>NNNFFDPKLMSDWEDEDLDTDNDNIPDSYERNGYTIKDLIAVKWEDSFAEQGYKKYVSNYLESNTAGDPYTDYEKASGSFDKAIKTEARDPLVAAYPIVGVGMEKLIISTNEHASTDQGKTVSRATTNSKTESNTAGVSVNVGYQNGFTANVTTNYSHTTDNSTAVQDSNGESWNTGLSINKGESAYINANVRYYNTGTAPMYKVTPTTNLVLDGDTLSTIKAQENQIGNNLSPGDTYPKKGLSPLALNTMDQFSSRLIPINYDQLKKLDAGKQIKLETTQVSGNFGTKNSSGQIVTEGNSWSDYISQIDSISASIILDTENESYERRVTAKNLQDPEDKTPELTIGEAIEKAFGATKKDGLLYFNDIPIDESCVELIFDDNTANKIKDSLKTLSDKKIYNVKLERGMNILIKTPTYFTNFDDYNNYPSTWSNVNTTNQDGLQGSANKLNGETKIKIPMSELKPYKRYVFSGYSKDPLTSNSIIVKIKAKEEKTDYLVPEQGYTKFSYEFETTEKDSSNIEITLIGSGTTYLDNLSITELNSTPEILDEPEVKIPTDQEIMDAHKIYFADLNFNPSTGNTYINGMYFAPTQTNKEALDYIQKYRVEATLQYSGFKDIGTKDKEMRNYLGDPNQPKTNYVNLRSYFTGGENIMTYKKLRIYAITPDDRELLVLSVD[7x];> APIERPEDFLKDKEKAKEWERKEAERIEQKLERSEKEALESYKKDSVEISKYSQTRNYFYDYQIEANSREKEYKELRNAISKNKIDKPMYVYYFESPEKFAFNKVIRTENQNEISLEKFNEFKETIQNKLFKQDGFKDISLYEPGKGDEKPTPLLMHLKLPRNTGMLPYTNTNNVSTLIEQGYSIKIDKIVRIVIDGKHYIKAEASVVSSLDFKDDVSKGDSWGKANYNDWSNKLTPNELADVNDYMRGGYTAINNYLISNGPVNNPNPELDSKITNIENALKREPIPTNLTVYRRSGPQEFGLTLTSPEYDFNKLENIDAFKSKWEGQALSYPNFISTSIGSVNMSAFAKRKIVLRITIPKGSPGAYLSAIPGYAGEYEVLLNHGSKFKINKIDSYKDGTITKLIVDATLIPENLYFQGL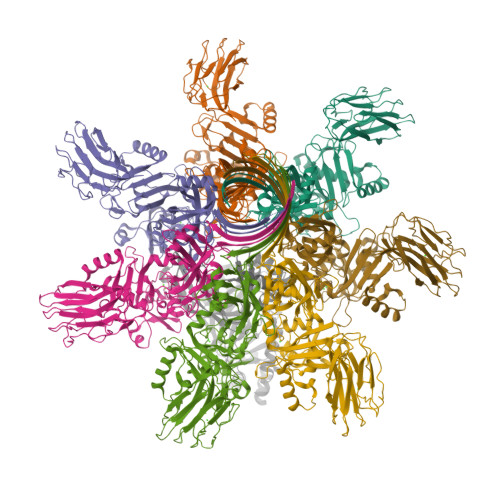EHHHHHH>MTIDLYYVPGSAPCRAVLLTAKALNLNLNLKLVDLHHGEQLKPEYLKLNPQHTVPTLVDDGLSIWESRAIITYLVNKYAKGSSLYPEDPKARALVDQRLYFDIGTLYQRFSDYFYPQVFAGAPADKAKNEKVQEALQLLDKFLEGQKYVAGPNLTVADLSLIASVSSLEASDIDFKKYANVKRWYETVKSTAPGYQEANEKGLEAFKGL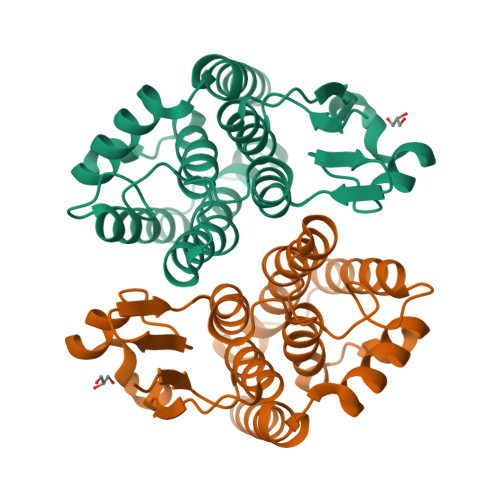VNSMLKK[4x]>GSPIKSRKGDVLHMHYTGKLEDGTEFDSSLPQNQPFVFSLGTGQVIKGWDQGLLGMCEGEKRKLVIPSELGYGERGAPPKIPGGATLVFEVELLKIE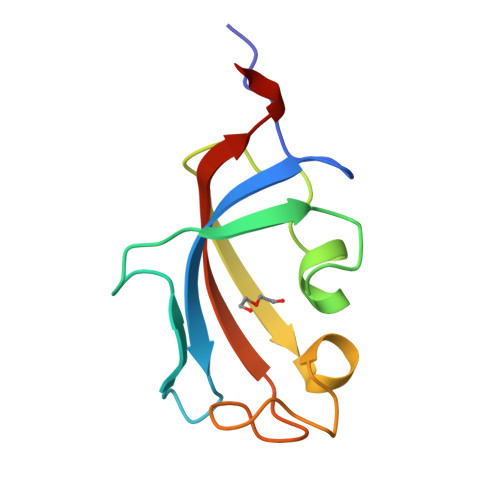RRTEL[4x]> AADAPAQLDPAGEKLYRSACVVCHASGV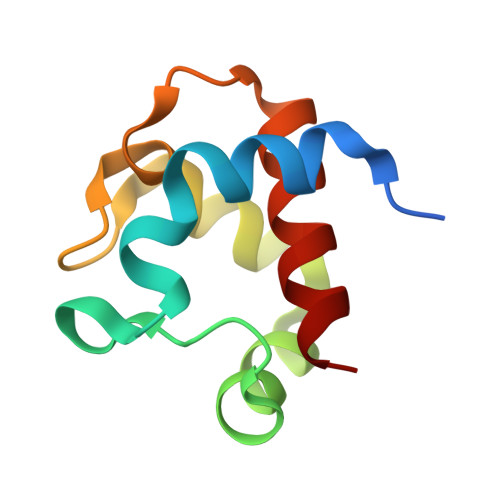ANAPKLGDKQAWAPFLAQGADALLATVLKGKGAMPPRGGTAADEATLRAAVAYMMDAAR> MSADSSPLVGSTPTGYGTLTIGTSIDPLSSSVSSVRLSGYCGSPWRVIGYHVVVWMMAGIPLLLFRWKPLWGVRLRLRPCNLAHAETLVIEIRDKEDSSWQLFTVQVQTEAIGEGSLEPSPQSQAEDGRSQAAVGAVPEGAWKDTAQLHKSEEAVSVGQKRVLRYYLFQGQRYIWIETQQAFYQVSLLDHGRSCDDVHRSRHGLSLQDQMVRKAIYGPNVISIPVKSYPQLLVDEALNPYYGFQAFSIALWLADHYYWYALCIFLISSISICLSLYKTRKQSQTLRDMVKLSMRVCVCRPGGEEEWVDSSELVPGDCLVLPQEGGLMPCDAALVAGECMVNESSLTGESIPVLKTALPEGLGPYCAETHRRHTLFCGTLILQARAYVGPHVLAVVTRTGFCTAKGGLVSSILHPRPINFKFYKHSMKFVAALSVLALLGTIYSIFILYRNRVPLNEIVIRALDLVTVVVPPALPAAMTVCTLYAQSRLRRQGIFCIHPLRINLGGKLQLVCFDKTGTLTEDGLDVMGVVPLKGQAFLPLVPEPRRLPVGPLLRALATCHALSRLQDTPVGDPMDLKMVESTGPQLQAMEEPPVPVSVLHRFPFSSALQRMSVVVAWPGATQPEAYVKGSPELVAGLCNPETVPTDFAQMLQSYTAAGYRVVALASKPLPTVPSLEAAQQLTRDTVEGDLSLLGLLVMRNLLKPQTTPVIQALRRTRIRAVMVTGDNLQTAVTVARGCGMVAPQEHLIIVHATGQPASLEFLPMESPTAVNGVKDPDQAASYTVEPDPRSRHLALSGPTFGIIVKHFPKLLPKVLVQGTVFARMAPEQKTELVCELQKLQYCVGMCGDGANDCGALKAADVGISLSQAEASVVSPFTSSMASIECVPMVIREGRCSLDTSFSVFKYMALYSLTQFISVLILYTINTNLGDLQFLAIDLVITTTVAVLMSRTGPALVLGRVRPPGALLSVPVLSSLLLQMVLVTGVQLGGYFLTLAQPWFVPLNRTVAAPDNLPNYENTVVFSLSSFQYLILAAAVSKGAPFRRPLYTNVPFLVALALLSSVLVGLVLVPGLLQGPLALRNITDTGFKLLLLGLVTLNFVGAFMLESVLDQCLPACLRRLRPKRASKKRFKQLERELAEQPWPPLPAGPLR

ATP13A2 belongs to the orphan P5B adenosine triphosphatases (ATPase) family and has been established as a lysosomal polyamine exporter to maintain the normal function of lysosomes and mitochondria. Here, using single-particle cryo-EM, we present the structures of full-length human ATP13A2 in three distinct conformations including an E1 state (apo), an E1P-ADP state with ATP and Mg2+, and an E2-Pi state with SPM, phosphatidic acid (PA), and phosphatidylinositol(3,5)bisphosphate [PI(3,5)P2]. The structure of the human ATP13A2 adopts the typical P-type ATPase fold with overall dimensions of 125 Å × 75 Å × 70 Å, including ten transmembrane (TM) helices and three conserved cytoplasmic domains [N (nucleotide-binding) domain; A (actuator) domain; and P (phosphorylation) domain]. In addition, the P5B type ATP13A2 also comprises two specific domains: a C-terminal extension domain (CTD) laying close to the P-domain and an N-terminal domain (NTD) preceding the A domain showing amphipathic feature.

To investigate the conformational change of ATP13A2 during the phosphorylation process, we solved two intermediate state structures, a 3.3 Å resolution E1 state and a 3.0 Å E1P-ADP state. Both of these two maps show well-resolved density. ATP binds to ATP13A2 and the resultant phosphoryl transfer reaction induces the rearrangement of the N domain, by which the N domain tilt around 30° to lay close to the A and P domain, thus sealing the crevice formed by the N and P domain compared to the E1 state. Notably, in our E1 state and E1P-ADP state structures, this cavity is nearly closed which prevents the binding and passage of substrate. The binding of ATP and Mg2+ induces the proximal arrangement of the N domain, by which the N domain tilt around 30° to lay close to the A and P domain, resulting in the E1-to-(E1-ATP) transition. Release of the Pi forms the intermediate E2 state, in which the cavity towards cytosol is open, thus allowing the translocation of SPM to the cytosol side. The A-domain should move back to the original position after the release of SPM to the cytosol, the protein then adopts the E1 conformation, ready to initiate another transport cycle.(2R,15R)-2-[(1-aminoisoquinolin-6-yl)amino]-8-fluoro-7-hydroxy-4,15,17-trimethyl-13-oxa-4,11-diazatricyclo[14.2.2.1~6,10~]henicosa-1(18),6(21),7,9,16,19-hexaene-3,12-dione 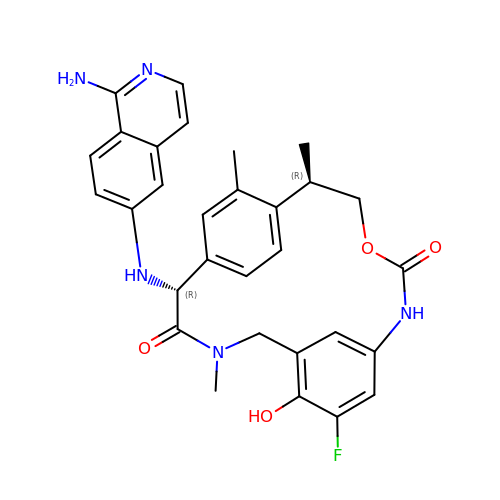| C30 H30 F N5 O4 | XABZFDVRWXGDRR-MRDQGFSESA-N>[4x]SMAKNRRDRNSWGGFSEKTYEWSSEEE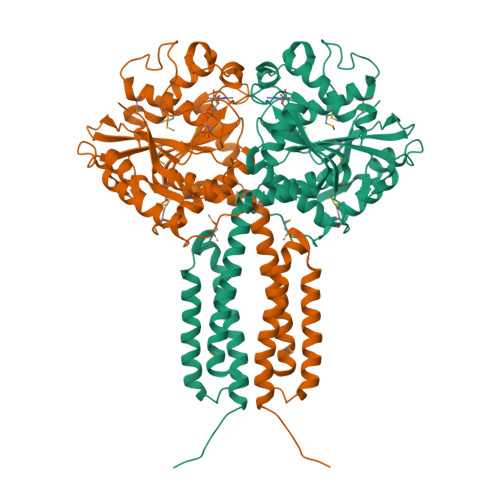EPVKKAGPVQVLIVKDDHSFELDETALNRILLSEAVRDKEVVAVSVAGAFRKGKSFLMDFMLRYMYNQESVDWVGDYNEPLTGFSWRGGSERETTGIQIWSEIFLINKPDGKKVAVLLMDTQGTFDSQSTLRDSATVFALSTMISSIQVYNLSQNVQEDDLQHLQLFTEYGRLAMEETFLKPFQSLIFLVRDWSFPYEFSYGADGGAKFLEKRLKVSGNQHEELQNVRKHIHSCFTNISCFLLPHPGLKVATNPNFDGKLKEIDDEFIKNLKILIPWLLSPESLDIKEINGNKITCRGLVEYFKAYIKIYQGEELPHPKSMLQATAEANNLAAVATAKDTYNKKMEEICGGDKPFLAPNDLQTKHLQLKEESVKLFRGVKKMGGEEFSRRYLQQLESEIDELYIQYIKHNDSKTIFHAAR> MGVVEEAHNVKVIGSGEATIVLGHGFGTDQSVWKHLVPHLVDDYRVVLYDNMGAGTTNPDYFDFDRY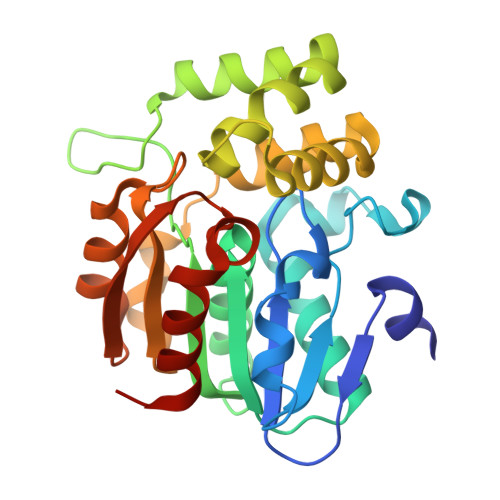SNLEGYSFDLIAILEDLKIESCIFVGHSVSAMIGVLASLNRPDLFSKIVMISASPRYVNDVDYQGGFEQEDLNQLFEAIRSNYKAWCLGFAPLAVGGDMDSIAVQEFSRTLFNMRPDIALSVGQTIFQSDMRQILPFVTVPCHILQSVKDLVVPVVVSEYLHANLGCESVVEVIPSDGHLPQLSSPDSVIPVILRHIRNDIAM> AKGTDSLKNSIEKYLKDKKAKVGVAVLGIEDNFKLNVNEKHHYPMQSTYKFHLALAVLDKLDKENISVDKKLFVKKSDLQPNTWSPLKDKY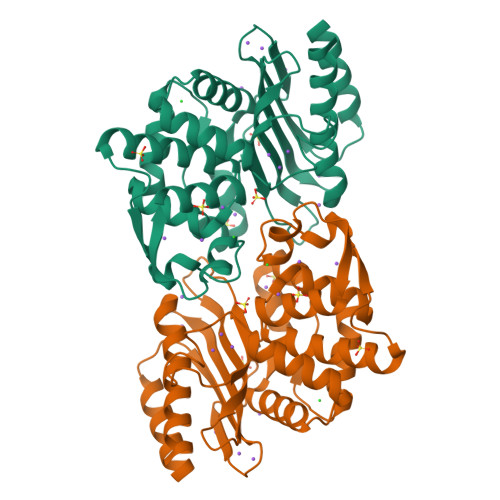PNGNLELSFSEIIKSTVSHSDNNGCDILFRFVGGTNKVHNFISKLGVKNISIKATEEEMHKAWNVQYTNWTTPDATVQLLKKFYKNEILSKNSYDFLLNTMIETTTGPKRLKGLLPDGTVVAHKTGSSDTNNKGITAATNDIGIITLPNGKHFAIAVYVSDSSEKSDVNEKIIAEICKSVWDYLVKDGK> MQNGVFTRENADFLVKSGADSPSSQSLLLRTSPSPLSLPRRRFIFLRSASVDLSERSSLACLAPFFCLASGVCLRSAFS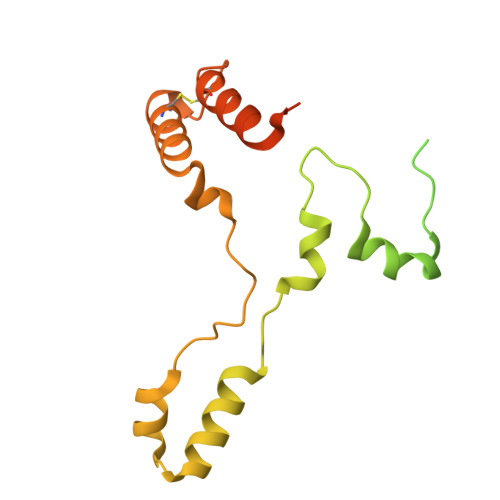LPFFARRGRPCLFFIFIFFFRVSFTANFRGKRVKMAASTIPISQWPSLLYAPPSSPANPAVEALPEMQFDDLHYPRQMLLCRGAGYSLEQCNRMAQPDARVTPENPAEKLLKEEAVAAIACLSQREGGKDEQCRYYIERMYKLANKEKQPEPGTLSKASTLACKLLGIHRPEA>[2x]MEQRITLKDYAMRFGQTKTAKDLGVYQSAINKAIHAGRKIFLTINADGSV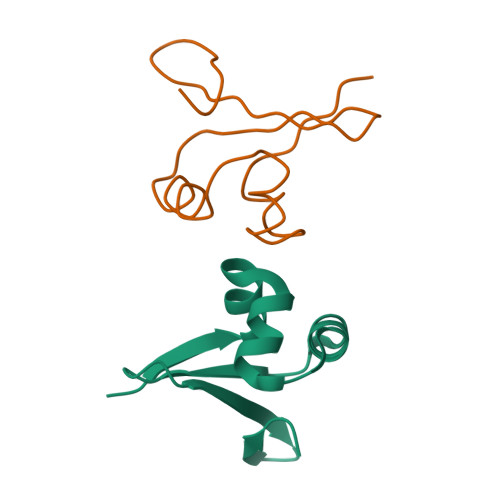YAEEVKDGEVKPWPS>DSLVFVQTDKSIYKPGQTVKFRVVSMDENFHPLNELIPLVYIQDPKGNRIAQWQSFQLEGGLKQFSFPLSSEPFQGSYKVVVQKKSGGRTE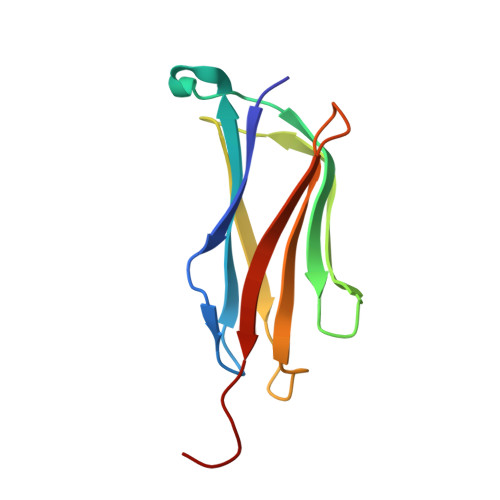HPFTVEEFVLP[2x]>QDSTSDLIPAPPLSKVPLQQNFQDNQFHGKWYVVGLAGNEVLREDKDPMKMWATIYELEEDKSYNVTIVMPLAEKCEYLFQTFVPGSQPGEFTLGGIKSGPGRTSGLVRVVSTNYNQHAMVFFKVVWQNREVFWVTLYGRTKELTSELKENFIRFSKSLGLPENHIVFPVPIDQCIDGSAWSHPQFEK[6x];>[6x]DTH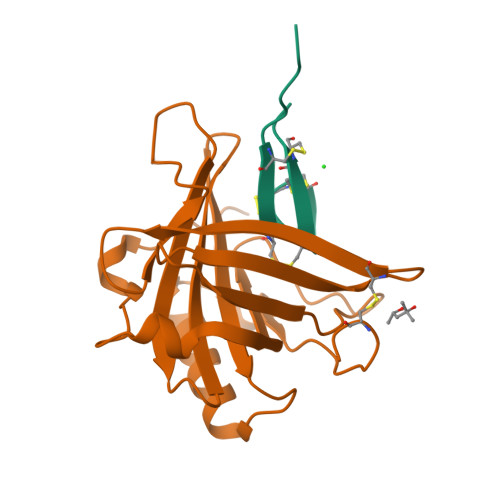FPICIFCCGCCHRSKCGMCCKT>GMEAHMKSHNLLEAVRFDDQRFVMELVHESENFKIVSFTFKAGQELPVHSHNIEGELNIVVLEGEGEFVGDGDAVIPAPRGAVLVAPIS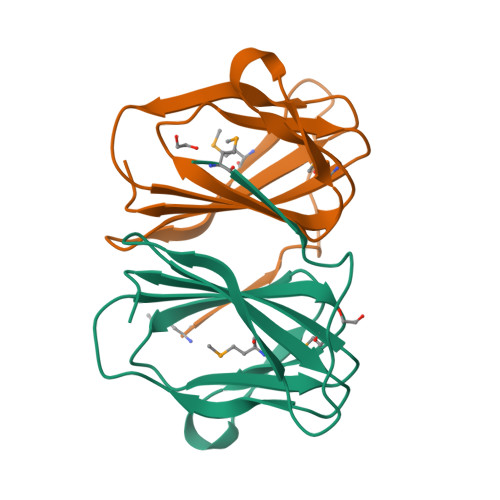TPHGVRAVTDMKVLVTIAPPI[8x]>[2x]PYASLTEIEHLVQSVCKSYRETCQLRLEDLLRQRSNIFSREEVTGYQRKSMWEMWERCAHHLTEAIQYVVEFAKRLSGFMELCQNDQIVLLKAGAMEVVLVRMCRAYNADNRTVFFEGKYGGMELFRALGCSELISSIFDFSHSLSALHFSEDEIALYTALVLINAHRPGLQEKRKVEQLQYNLELAFHHHLCKTHRQSILAKLPPKGKLRSLCSQHVERLQIFQ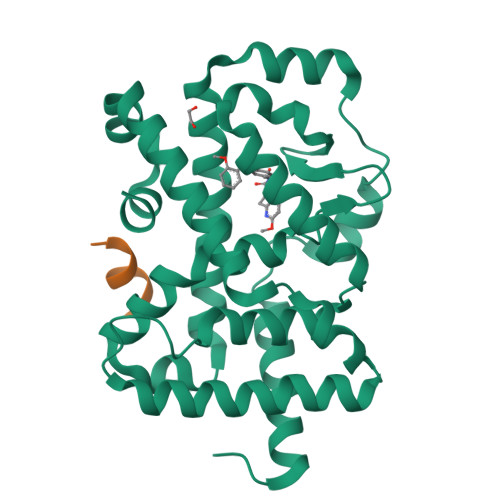HLHPIVVQAAFPPLYKELFS;>[2x]KILHRLLQ> MAAPQFHRPSTITADNVRALGMRGLVLATNNAQFIMDNSYPHPHGTQGAVREFLRGQAAALTDLGVTHANNTFAPQPMFAGDAAAEWLRPSFGLKRTYSPFVVRDPK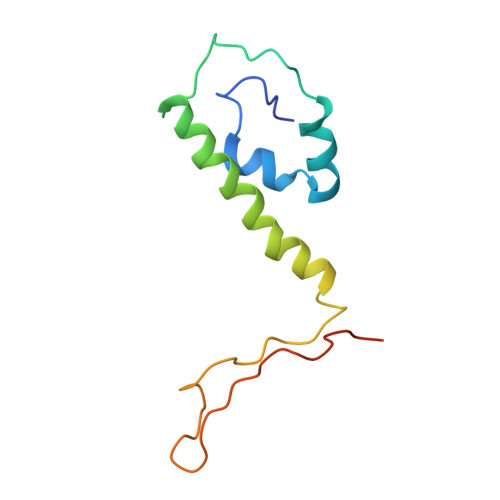TPSTP> PGLAYGNPYSG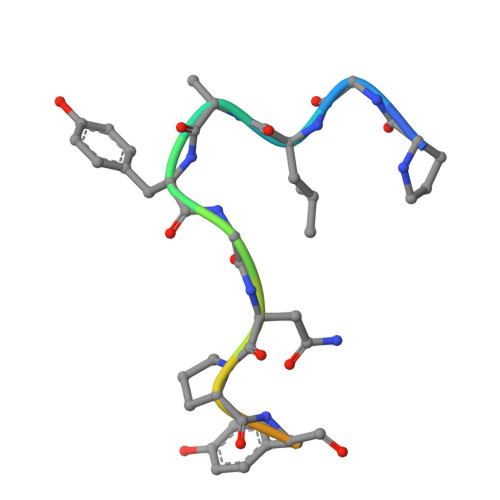IQE2-[4-[2-fluoranyl-5-[3-(6-methylpyridin-2-yl)-1~{H}-pyrazol-4-yl]phenyl]phenyl]sulfonylethanol | C23 H20 F N3 O3 S 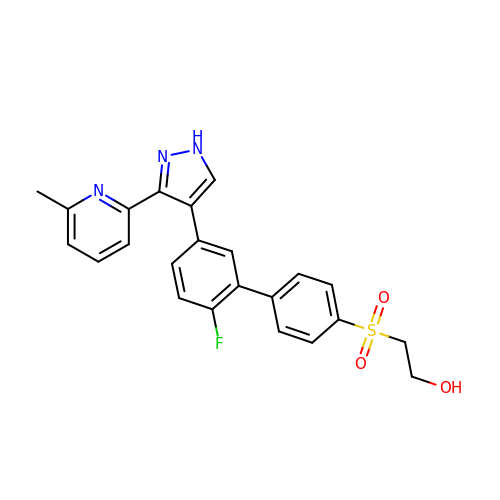| IFQCNLVDAWIXAR-UHFFFAOYSA-N>[4x]SMKLDIKKTFSNRSDRVKGIDFHPTEPWVLTTLYSGRVEIWNYETQVEVRSIQVTETPVRAGKFIARKNWIIVGSDDFRIRVFNYNTGEKVVDFEAHPDYIRSIAVHPTKPYVLSGSDDLTVKLWNWENNWALEQTFEGHEHFVMCVAFNPKDPST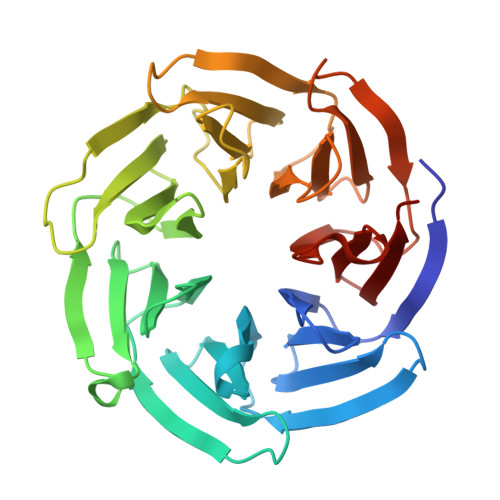FASGCLDRTVKVWSLGQSTPNFTLTTGQERGVNYVDYYPLPDKPYMITASDDLTIKIWDYQTKSCVATLEGHMSNVSFAVFHPTLPIIISGSEDGTLKIWNSSTYKVEKTLNVGLERSWCIATHPTGRKNYIASGFDNGFTVLSLG> KYKALAREAALSKIGELASEIFAEFTEGKYSEVVVRAEEN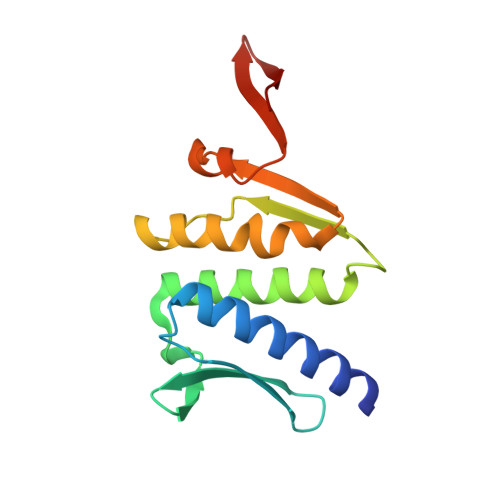KVRLFVVWEGKERPLTFLSGGERIALGLAFRLAMSLYLAGEISLLILDEPTPYLDEERRRKLITIMERYLKKIPQVILVSHDEELKDAADHVIRISLENGSSKVEVVS> T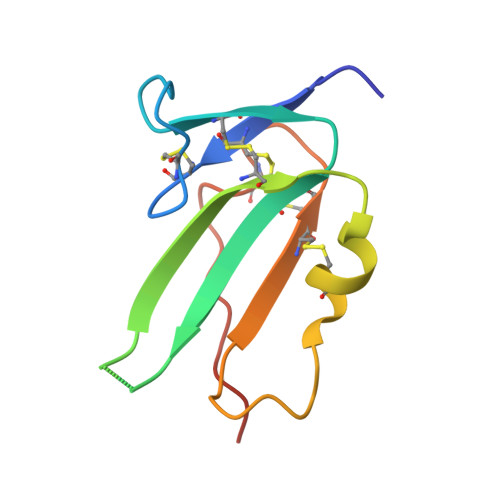LPFLKCYCSGHCPDDAINNTCITNGHCFAIIEEDDQGETTLASGCMKYEGSDFQCKDSPKAQLRRTIECCRTNLCNQYLQPTLPPVVI>SNAARDNVTKSKISQYKDQIFDLTYPYSGNENSSVIAVGFLDYSCGHCKAIKNDIKQLINDGKIKYIFRDAPILGNASLKAAKSALAVYFLDKEKYFDFHHAALSHKGEFSDESILDIVKNIGIDEDDFNDSIKDNADKIEQMINNSRLLVRDLGVGGTPFLIIGDSLFVGATDLNVLRKKVDELSHKQG[4x]

The introduction, isomerization and reduction of protein disulfide bonds in bacteria are controlled by disulfide-bond-forming (DSB) proteins. wMel strain encodes two DsbA-like proteins, α-DsbA1 and α-DsbA2, and the integral membrane protein α-DsbB. In contrast, α-DsbA2, which is highly conserved in Wolbachia, does not interact with α-DsbB and has a long N-terminal region compared with α-DsbA1. Our results show that FL α-DsbA2 is a strong protein disulfide isomerase and that the removal of the N-terminal residues eliminates this activity but gives rise to weak dithiol oxidase activity.

We used two constructs: (i) FL α-DsbA2, the full-length mature α-DsbA2 (lacking the signal peptide that directs the protein to the periplasm) comprising residues 16–252, and (ii) α-DsbA2ΔN, a truncated form of α-DsbA2 (lacking both the signal sequence and the 50-residue N-terminal region) comprising residues 65–252. We were unable to generate crystals of full-length mature α-DsbA2. The crystal structure of truncated α-DsbA2ΔN reveals a classic monomeric DsbA-like architecture. Using SAXS data, the molecular mass of truncated α-DsbA2ΔN was estimated to be ∼23 kDa from I(0) and the Porod volume, which is very close to the expected mass for an α-DsbA2ΔN monomer (21 kDa) and is consistent with the crystal structure that we report here. We next assessed the protein disulfide isomerase activity of FL α-DsbA2 and α-DsbA2ΔN by following the reactivation of scrambled RNase A in an in vitro assay. By comparison, truncated α-DsbA2ΔN recovered just 35 ± 3% of the RNase A activity relative to native refolded RNase A over this period, similar to that reported for the oxidase enzyme EcDsbA. Therefore, we conclude that α-DsbA2 is a protein disulfide isomerase and that its disulfide isomerase activity requires the presence of the N-terminal residues. Notably, there is a basic region near the catalytic site of both PmScsC and EcDsbC that is absent in α-DsbA2. A hydrophobic region is also present in PmScsC and EcDsbC, and the conservation of this feature suggests this is a binding site for unfolded protein substrates.>MGRIKNKQFAVIGLGRFGGSIVKELHRMGHEVLAVDINEEKVNAYASYATHAVIANATEENELLSLGIRNFEYVIVAIGANIQASTLTTLLLKELDIPNIWVKAQNYYHHKVLEKIGADRIIHPEKDMGVKIAQ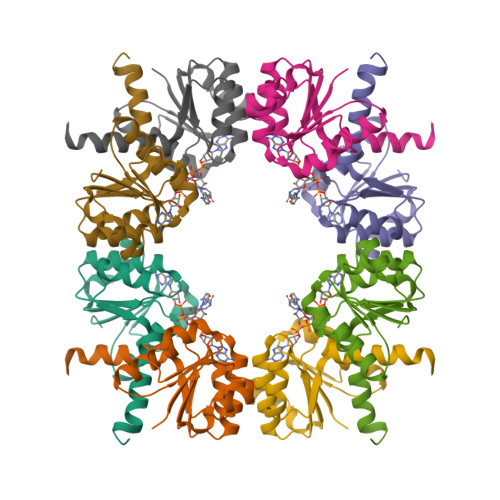SLSDENVLNY[2x]> MLGTGPAAATTAATTSXXXXXXXXXXXXXXSRNEETXXXXXXXXXXXXXXXXXEMSQEESTRFYDQLNHHIFELVSSSDANERKGGILAIASLIGVEGGNATRIGRFANYLRNLLPSNDPVVMEMASKAIGRLAMAGDTFTAEYVEFEVKRALEWLGADRNEGRRHAAVLVLRELAISVPTFFFQQVQPFFDNIFVAVWDPKQAIREGAVAALRACLILTTQREPKEMQKPQWYRHTFEEAEKGFDETLAKEKGMNRDDRIHGALLILNELVRISSMEGERLREEMEEITQQQLVHDKYCKDLMGFGTKPRHITPFTSFQAVQPQQSNALVGLLGYSSHQGLMGFGTSPSPAKSTXXXXXXXXXXXXXXXXXXXXXXXXXRNSKNSLIQMTILNLLPRLAAFRPSAFTDTQYLQDTMNHVLSCVKKEKERTAAFQALGLLSVAVRSEFKVYLPRVLDIIRAALPPKDFAHKRQKAMQVDATVFTCISMLARAMGPGIQQDIKELLEPMLAVGLSPALTAVLYDLSRQIPQLKKDIQDGLLKMLSLVLMHKPLRHPGMPKGLAHQLASPGLTTLPEASDVGSITLALRTLGSFEFEGHSLTQFVRHCADHFLNSEHKEIRMEAARTCSRLLTPSIHLISGHAHVVSQTAVQVVADVLSKLLVVGITDPDPDIRYCVLASLDERFDAHLAQAENLQALFVALNDQVFEIRELAICTVGRLSSMNPAFVMPFLRKMLIQILTELEHSGIGRIKEQSARMLGHLVSNAPRLIRPYMEPILKALILKLKDPDPDPNPGVINNVLATIGELAQVSGLEMRKWVDELFIIIMDMLQDSSLLAKRQVALWTLGQLVASTGYVVEPYRKYPTLLEVLLNFLKTEQNQGTRREAIRVLGLLGALDPYKHKVNIGMIDQSRDASAVSLSESKSSQDSSDYSTSEMLVNMGNLPLDEFYPAVSMVALMRIFRDQSLSHHHTMVVQAITFIFKSLGLKCVQFLPQVMPTFLNVIRVCDGAIREFLFQQLGMLVSFVKSHIRPYMDEIVTLMREFWVMNTSIQSTIILLIEQIVVALGGEFKLYLPQLIPHMLRVFMHDNSPGRIVSIKLLAAIQLFGANLDDYLHLLLPPIVKLFDAPEAPLPSRKAALETVDRLTESLDFTDYASRIIHPIVRTLDQSPELRSTAMDTLSSLVFQLGKKYQIFIPMVNKVLVRHRINHQRYDVLICRIVKGYTLADEEEDPLIYQHRMLRSGQGDALASGPVETGPMKKLHVSTINLQKAWGAARRVSKDDWLEWLRRLSLELLKDSSSPSLRSCWALAQAYNPMARDLFNAAFVSCWSELNEDQQDELIRSIELALTSQDIAEVTQTLLNLAEFMEHSDKGPLPLRDDNGIVLLGERAAKCRAYAKALHYKELEFQKGPTPAILESLISINNKLQQPEAAAGVLEYAMKHFGELEIQATWYEKLHEWEDALVAYDKKMDTNKDDPELMLGRMRCLEALGEWGQLHQQCCEKWTLVNDETQAKMARMAAAAAWGLGQWDSMEEYTCMIPRDTHDGAFYRAVLALHQDLFSLAQQCIDKARDLLDAELTAMAGESYSRAYGAMVSCHMLSELEEVIQYKLVPERREIIRQIWWERLQGCQRIVEDWQKILMVRSLVVSPHEDMRTWLKYASLCGKSGRLALAHKTLVLLLGVDPSRQLDHPLPTVHPQVTYAYMKNMWKSARKIDAFQHMQHFVQTMQQQAQHAIATEDQQHKQELHKLMARCFLKLGEWQLNLQGINESTIPKVLQYYSAATEHDRSWYKAWHAWAVMNFEAVLHYKHQNQARDEKKKLRHASGANITNATTAATTAATATTTASTEGSNSESEAESTENSPTPSPLQKKVTEDLSKTLLMYTVPAVQGFFRSISLSRGNNLQDTLRVLTLWFDYGHWPDVNEALVEGVKAIQIDTWLQVIPQLIARIDTPRPLVGRLIHQLLTDIGRYHPQALIYPLTVASKSTTTARHNAANKILKNMCEHSNTLVQ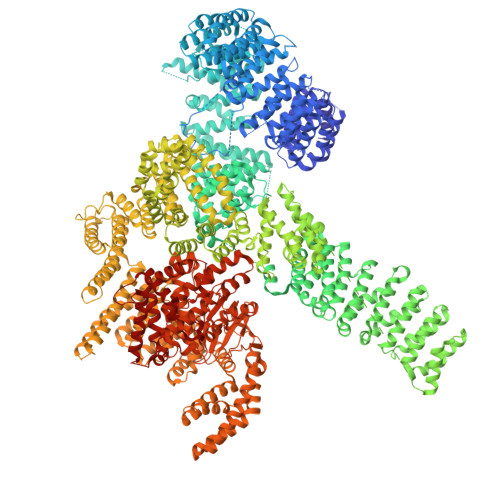QAMMVSEELIRVAILWHEMWHEGLEEASRLYFGERNVKGMFEVLEPLHAMMERGPQTLKETSFNQAYGRDLMEAQEWCRKYMKSGNVKDLTQAWDLYYHVFRRISKQLPQLTSLELQYVSPKLLMCRDLELAVPGTYDPNQPIIRIQSIAPSLQVITSKQRPRKLTLMGSNGHEFVFLLKGHEDLRQDERVMQLFGLVNTLLANDPTSLRKNLSIQRYAVIPLSTNSGLIGWVPHCDTLHALIRDYREKKKILLNIEHRIMLRMAPDYDHLTLMQKVEVFEHAVNNTAGDDLAKLLWLKSPSSEVWFDRRTNYTRSLAVMSMVGYILGLGDRHPSNLMLDRLSGKILHIDFGDCFEVAMTREKFPEKIPFRLTRMLTNAMEVTGLDGNYRITCHTVMEVLREHKDSVMAVLEAFVYDPLLNWRLMDTNTKGNKRSRTRTDSYSAGQSVEILDGVELGEPAHKKTGTTVPESIHSFIGDGLVKPEALNKKAIQIINRVRDKLTGRDFSHDDTLDVPTQVELLIKQATSHENLCQCYIGWCPFW>MTKQHAFTREDLLRCSR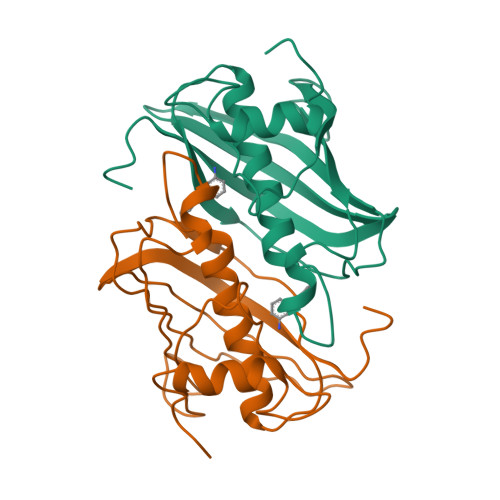GELFGPGNAQLPAPNMLMIDRIVHISDVGGKYGKGELVAELDINPDLWFFACHFEGDPVMPGCLGLDAMWQLVGFYLGWQGNPGRGRALGSGEVKFFGQVLPTAKKVTYNIHIKRTINRSLVLAIADGTVSVDGREIYSAEGLRVGLFTSTDSF[2x]> AEEAFD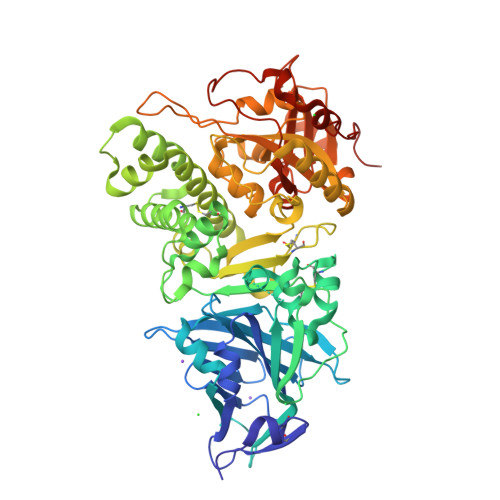LWNECAKACVLDLKDGVRSSRMSVDPAIADTNGQGVLHYSMVLEGGNDALKLAIDNALSITSDGLTIRLEGGVEPNKPVRYSYTRQARGSWSLNWLVPIGHEKPSNIKVFIHELNAGNQLSHMSPIYTIEMGDELLAKLARDATFFVRAHESNEMQPTLAISHAGVSVVMAQAQPRREKRWSEWASGKVLCLLDPLDGVYNYLAQQRCNLDDTWEGKIYRVLAGNPAKHDLDIKPTVISHRLHFPEGGSLAALTAHQACHLPLETFTRHRQPRGWEQLEQCGYPVQRLVALYLAARLSWNQVDQVIRNALASPGSGGDLGEAIREQPEQARLALTLAAAESERFVRQGTGNDEAGAANADVVSLTCPVAAGECAGPADSGDALLERNYPTGAEFLGDGGDVSFSTRGTQNWTVERLLQAHRQLEERGYVFVGYHGTFLEAAQSIVFGGVRARSQDLDAIWRGFYIAGDPALAYGYAQDQEPDARGRIRNGALLRVYVPRSSLPGFYRTSLTLAAPEAAGEVERLIGHPLPLRLDAITGPEEEGGRLETILGWPLAERTVVIPSAIPTDPRNVGGDLDPSSIPDKEQAISALPDYASQPGKPPREDLK> MESGELIKRLEDAGWQIRGGRKTNSGSHVTLCKPG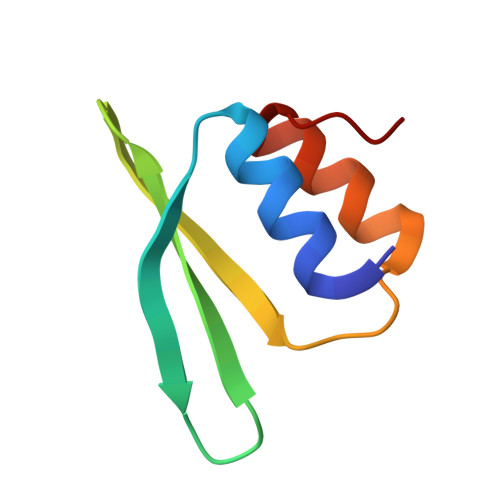VRKIITLPYPRKDISKGLLRQAQKIAGIKLS>[4x]MKEIKLILTDIDGVWTDGGMFYDQTGNE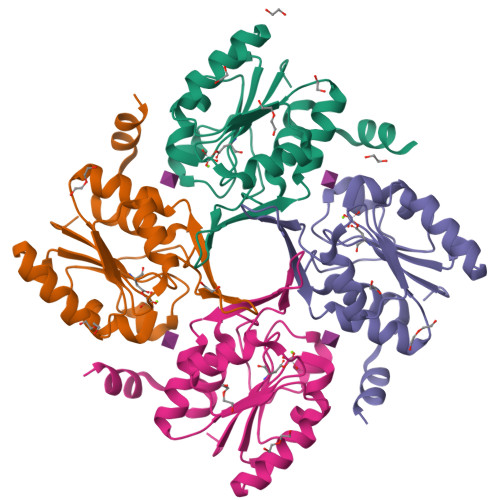WKKFNTSDSAGIFWAHNKGIPVGILTGEKTEIVRRRAEKLKVDYLFQGVVDKLSAAEELCNELGINLEQVAYIGDDLNDAKLLKRVGIAGVPASAPFYIRRLSTIFLEKRGGEGVFREFVEKVLGINLEDFIAVIQ>[4x]MAHHHHHHSLSSPNLSFYYNECERFESFLKNHHLHLESFHPYLEKAFFEMVLNGGKRFRPKLFLAVLCALVGQKDYSNQQTEYFKIALSIECLHTYSLIHDDLPCMDNAALRRNHPTLHAKYDETTAVLIGDALNTYSFELLSNALLESHIIVELIKILSANGGIKGMILGQALDCYFENTPLNLEQLTFLHEHKTAKLISASLIMGLVASGIKDEELFKWLQAFGLKMGLCF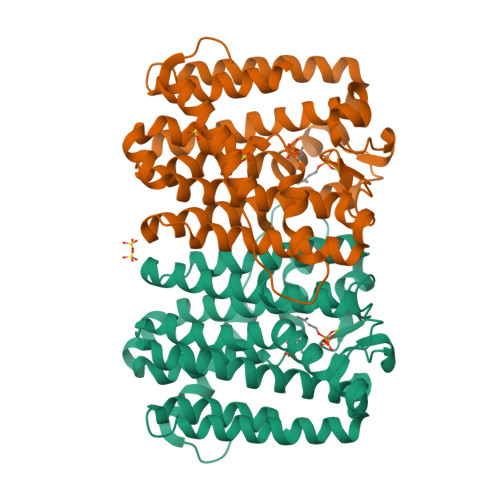QVLDDIIDVTQDEEESGKTTHLDSAKNSFVNLLGLERANNYAQTLKTEVLNDLDALKPAYPLLQENLNALLNTLFKG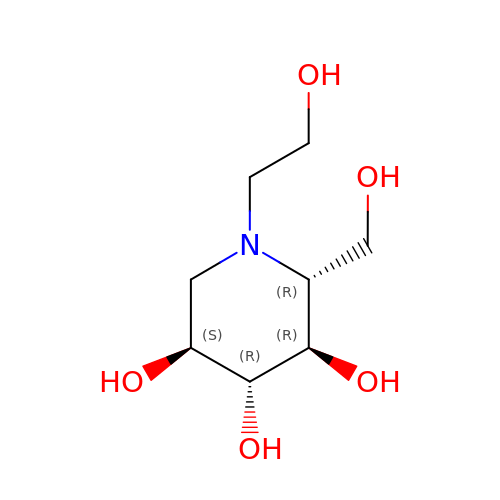(2R,3R,4R,5S)-1-(2-hydroxyethyl)-2-(hydroxymethyl)piperidine-3,4,5-triol | C8 H17 N O5 | IBAQFPQHRJAVAV-ULAWRXDQSA-N> NREEKILNREIGFAIGMPVCEFDMVKDPEVQDFRRNILNVCKEAVDLRDLNSPHSRAMYVYPPNVESSPELPKHIYNKLDKGQIIVVIWVIVSPNNDKQKYTLKINHDCVPEQVIAEAIRKKTRSMLLSSEQLKLCVLEYQGKYILKVCGCDEYFLEKYPLSQYKYIRSCIMLGRMPNLMLMAKESLYSQLPMDCFTMPSYSRRISTATPYMNGETSTKSLWVINSALRIKILCATYVNVNIRDIDKIYVRTGIYHGGEPLCDNVNTQRVPCSNPRWNEWLNYDIYIPDLPRAARLCLSICSVKGRKGAKEEHCPLAWGNINLFDYTDTLVSGKMALNLWPVPHGLEDLLNPIGVTGSNPNKETPCLELEFDWFSSVVKFPDMSVIEEHANWSVSREAGFSYSHAGLSNRLARDNELRENDKEQLKAISTRDPLSEITEQEKDFLWSHRHYCVTIPEILPKLLLSVKWNSRDEVAQMYCLVKDWPPIKPEQAMELLDCNYPDPMVRGFAVRCLEKYLTDDKLSQYLIQLVQVLKYEQYLDNLLVRFLLKKALTNQRIGHFFFWHLKSEMHNKTVSQRFGLLLESYCRACGMYLKHLNRQVEAMEKLINLTDILKQEKKDETQKVQMKFLVEQMRRPDFMDALQGFLSPLNPAHQLGNLRLEECRIMSSAKRPLWLNWENPDIMSELLFQNNEIIFKNGDDLRQDMLTLQIIRIMENIWQNQGLDLRMLPYGCLSIGDCVGLIEVVRNSHTIMQIQCKGGLKGALQFNSHTLHQWL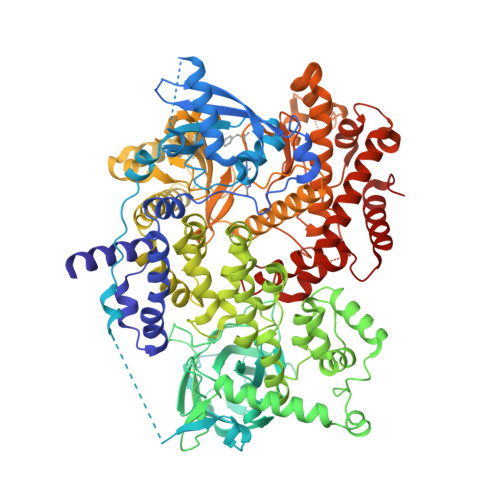KDKNKGEIYDAAIDLFTRSCAGYCVATFILGIGDRHNSNIMVKDDGQLFHIDFGHFLDHKKKKFGYKRERVPFVLTQDFLIVISKGAQECTKTREFERFQEMCYKAYLAIRQHANLFINLFSMMLGSGMPELQSFDDIAYIRKTLALDKTEQEALEYFMKQMNDAHHGGWT>[4x]SMGVRKLATIRTAGEITPIAGAEAIECCHVDGWTCVIKKGEFKQGDRGVYFEIDSFIKEDNDRYPMLSKQVIDYEGQRGTRLRTARLRGQLSQGLFLPMDRFPELASNQVGDDVTEILGITKWEPPISTNLSGEILGEFPTFISKTDQERVQNLIPQIEENKGQKFEVTVKLAGSSMTVYRKDDHIGVCGRNWELRETATNAQW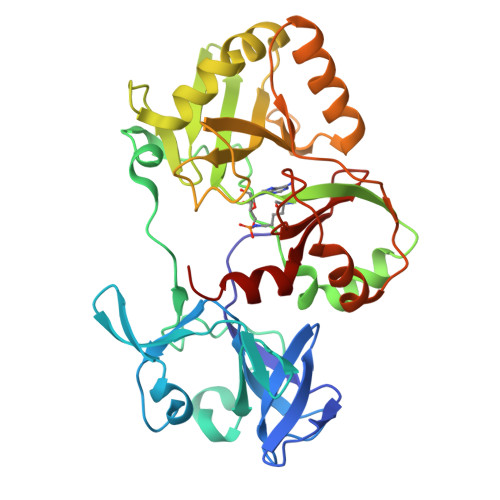HAARRNKMIEGLQFLNRNLALQGEIIGESIQGNLEKLKGQDFYLFDIYDIDKAQYLTPIERQSLVKQLNDNGFTVKHVPILDDLELNHTAEQILAMADGPSLNKNVKREGLVFKRLDGKFSFKAISNAYLEKHKDR> ALEGTEFARSEGASALASVNPLKTTVEEALS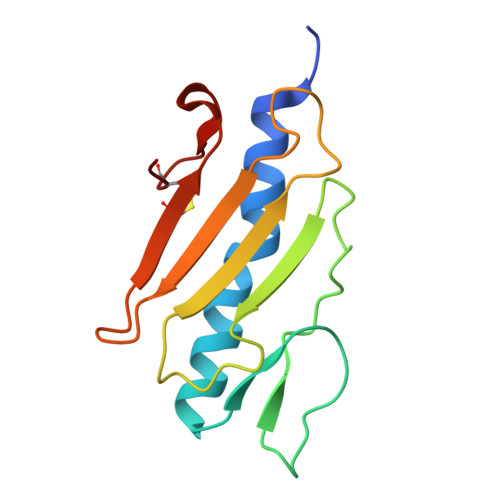RGWSVKSGTGTEDATKKEVPLGVAADANKLGTIALKPDPADGTADITLTFTMGGAGPKNKGKIITLTRTAADGLWKCTSDQDEQFIPKGCSR>[12x]PRSLANAPIMILNGPNLNLLGQAQPEIYGSDTLADVEALCVKAAAAHGGTVDFRQSNHEGELVDWIHEARLNHCGIVINPAAYSHTSVAILDALNTCDGLPVVEVHI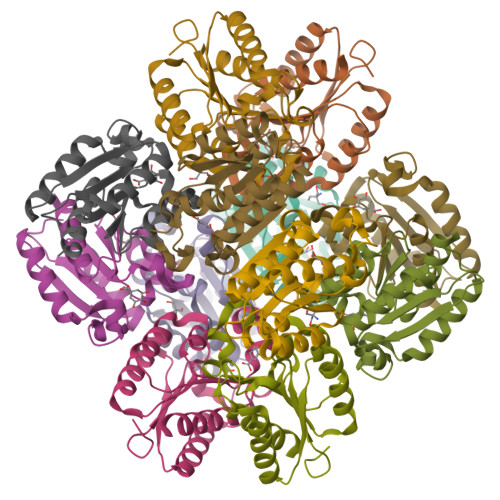SNIHQREPFRHHSYVSQRADGVVAGCGVQGYVFGVERIAALAGAGSARA>[2x]MKFGINLFPTVGPAEKSAGQHFEESLRLAELADELGFHHVKTVEHYFHEYGGYSPDPVTFLAAAAARTRRVRLVTGAVLPVFTHPLKLAGKLAMLDNISQGRLDVGFGRAFLPDEFTAFEISMDESRARFDEGVEAVRRLWAEEDVVWEGTFHRFGPVTMLPRTWQRPHPRILVATAKTPASAEAAARAGHGVMLVPSINPREQVQKTLSLYRDAASAAGFKPTEEDIHMSYNCYLAEDGQEARQKGGQASERANRALASAVSAWRETRSADYPGYEKIVEKAGRGDFDRAVAERKALVGTPDEVRAAIDDIRGWFGDFTISLQVISGAMPFEESARTMRLFAEHLLPHYAAND

Rishirilides are a group of PKS II secondary metabolites produced by Streptomyces bottropensis Gö C4/4. Structurally, rishirilide is a tricyclic partially aromatic polyketide with an unusual isopentyl sidechain and a carbonyl group on the third ring. In this study the involvement of one cyclase and two oxygenase in rishirilide biosynthesis was investigated. For this purpose, excision of rslC3 gene using the markerless time-saving CRISPR-Cas9 system, inactivation of rslO4 gene using Redirect® technology, and crystallization of RslO4 and RslO1 proteins were carried out.

The monooxygenase RslO1 crystallizes as a homodimer and the overall structure of each subunit is made up of a well-conserved 8 β-strands TIM-barrel surrounded by 8 α-helixes. Each β-strand connects an α-helix through a short loop region. According to the structural homology study using Swiss Model Server, RslO1 was revealed to be FMN-dependent bacterial luciferase-like monooxygenase. RslO1 belongs to the family of FMN-dependent luciferase-like monooxygenases. The RslO1 three-dimensional structure shows a high similarity to FMN-dependent luciferase-like monooxygenases such as the epoxy-forming MsnO8 which acts with the flavin reductase MsnO3 in mensacarcin biosynthesis in the same strain. The high similarity in three-dimensional structure between RslO1 and the epoxy-forming MsnO8 enzyme in mensacarcin biosynthesis in S. bottropensis indicates a similar activity of RslO1 enzyme in the epoxide formation to form RslO5-substrate during rishirilide biosynthesis in the same strain. According to the high sequence identity between RslO2 and MsnO3 (47%), it is most likely that RslO2 acts as flavin reductase, by using NADH as a hydrogen source, to provide RslO1 with the reduced FMN in a similar mechanism of MsnO8-MsnO3 two-component epoxide-forming system. In his turn the FMN-dependent luciferase-like monooxygenase RslO1 is responsible for the formation of an epoxide providing a substrate for RslO5. Following the epoxidation mediated by RslO1-RslO2 system, RslO1 product undergoes an epoxide reduction by RslO5 and then oxidative carbon backbone rearrangement including RslO9-mediated Baeyer–Villiger oxidation and lactone formation.> YDPFGG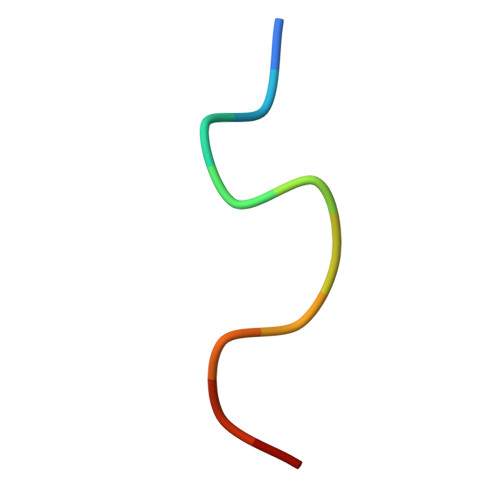DPFKG4-({(2S)-2-[2-(4-chlorophenyl)-5,6-difluoro-1H-benzimidazol-1-yl]-2-cyclohexylacetyl}amino)-3-methylbenzoic 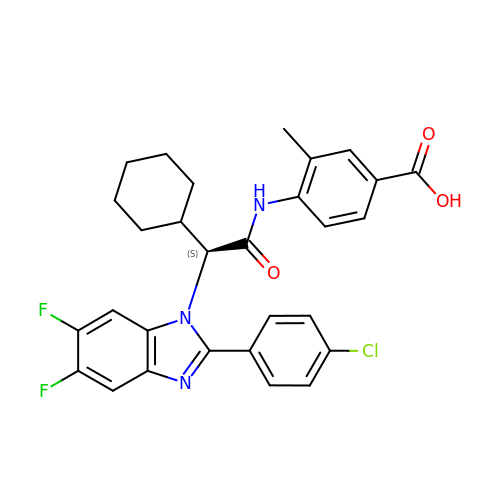acid | C29 H26 Cl F2 N3 O3 | XAVJTYOBWCSWFJ-SANMLTNESA-N> TKKGATKILFIYKLS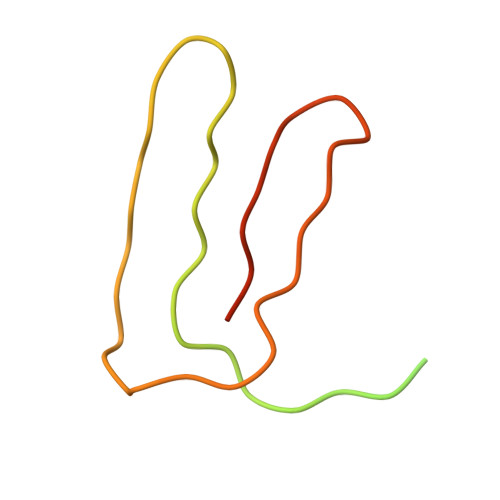KLNVYNNESYKIKLLFNHLYCIDNYNSIYFNLNGILIWLNVLHINIILIKYAFLILLNNLEYLIIFKYNIISIK>[4x]MAREFKSKNFWKAVLAELVGMTLFIFLSLSAAIGNKNSTNPDQEVKVSLAFGLAIATLAQSLGHISGAHLNPAVTLGMLASCQISVLKAVMY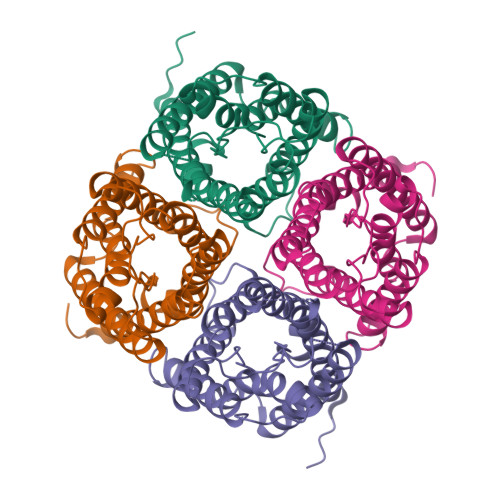IVAQMLGSALASGIVYGTRPNGNANLGLNALSGVTPSQGVGIELLATFQLVLCVIAVTDKRRRDVTGSAPLAIGLSVCLGHLAAISYTGCGINPARSFGPALILNNFENHWVYWVGPMCGGVAAALIYDFLLAPKFDDFPERIKVLVSGPVG> MGSDKIHHHHHHRTKDQYYELRDFALGTSVRIVVSSQKINPRTIAEAILEDMKRITYKFSFTDERSVVKKINDHPNEWVEVDEETYSLIKAACAFAELTDGAFDPTVGRLLELWGFTGNYENLRVPSREEIEEALKHTGYKNVLFDDKNMRVMVKNGVK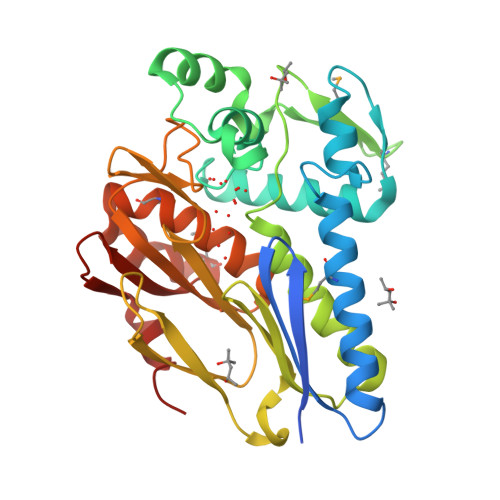IDLGGIAKGYALDRARQIALSFDENATGFVEAGGDVRIIGPKFGKYPWVIGVKDPRGDDVIDYIYLKSGAVATSGDYERYFVVDGVRYHHILDPSTGYPARGVWSVTIIAEDATTADALSTAGFVMAGKDWRKVVLDFPNMGAHLLIVLEGGAIERSETFKLFERE>[3x]MAILTDENYVDKAERAISLLEKDNKGNYLLTTSQIRKLLSLCSSLYDRSKERKFDELINDVSYLRVQFVYQAGREIAVKDLIEKAQILEALKEIKDRETLQRFCRYMEALVAYFKFYGGKD;>[5x]MTFAKIKFSAQIRLETGLHIGGSDAFAAIGAIDSPVIKDPITNIPIIPGSSLKGKMRTLLAKVYNEKVAEKPSDDSDILSRLFGNSKDKRFKMGRLIFRDAFLSNADELDSLGVRSYTEVKFENTIDRITAEANPRQIERAIRNSTFDFELIYEITDENENQVEEDFKVIRDGLKLLELDYLGGSGSRGYGKVAFEKLKATTVFGNYDVKTLNELLTAEV;> MTYKLYIMTFQNAHFGSGTLDSSKLTFSADRIFSALVLESLKMGKLDAFLAEANQDKFTLTDAFPFQFGPFLPKPIGYPKHDQIDQSVDVKEVRRQAKLSKKLQFLALENVDDYLNGELFENEEHAVIDTVTKNQPHKDGNLYQVATTRFSNDTSLYVIANESDLLNELMSSLQYSGLGGKRSSGFGRFELDIQNIPLELSDRLTKNHSDKVMSLTTALPVDADLEEAMEDGHYLLTKSSGFAFSHATNENYR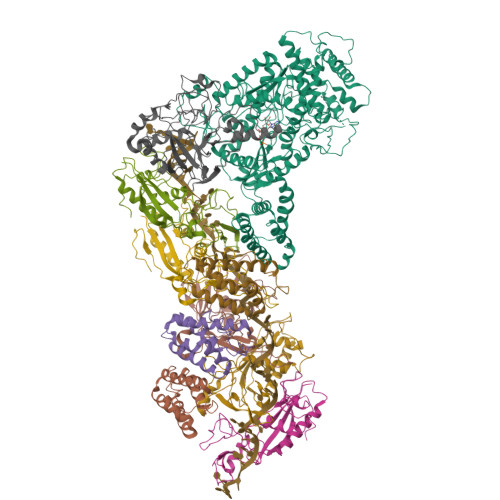KQDLYKFASGSTFSKTFEGQIVDVRPLDFPHAVLNYAKPLFFKLEV;> MKKEKIDLFYGALLHDIGKVIQRATGERKKHALVGADWFDEIADNQVISDQIRYHMANYQSDKLGNDHLAYITYIADNIASGVDRRQSNEESDEDASAKIWDTYTNQADIFNVFGAQTDKRYFKPTVLNLKSKPNFASATYEPFSKGDYAAIATRIKNELAEFEFNQAQIDSLLNLFEAILSFVPSSTNSKEIADISLAEHSRLTAAFALAIYDYLEDKGRHNYKEDLFTKASAFYEEEAFLLASFDLSGIQDFIYNIATSGAAKQLKARSLYLDFMSEYIADSLLDKLGLNRANLLYVGGGHAYFVLANTEKTVETLVQFEKDFNQFLLANFQTRLYVAFGWGSFAAKDIMSELNSPESYRQIYQKASRMISEKKISRYDYRTLMLLNRGGKSSERECEICHSVENLVSYHDQKVCDICRGLYQFSKEIAHDHFIITENEGLPIGPNACLKGVAFEKLSQESFSRVYVKNDYKAGTIKATHVFVGDYQCDEIHKYAALSKNEDGLGIKRLAVVRLDVDDLGAAFMAGFSRQGNGQYSTLSRSATFSRSMSLFFKVYINQFASDKKLSIIYAGGDDVFAIGSWQDIIAFTVELRQNFIKWTNGKLTLSAGIGLFADKTPISLMAHQTGELEEAAKGNEKDSISLFSSDYTFKFDRFITNVYDDKLEQIRYFFNHQDERGKNFIYKLIELLRNYESEEKMNVARLAYYLTRLEELTDKDERDKFKQFKKLFFKWYTNNESDRKEAELALLLYVYEIRKD>CGGCGGCCGC[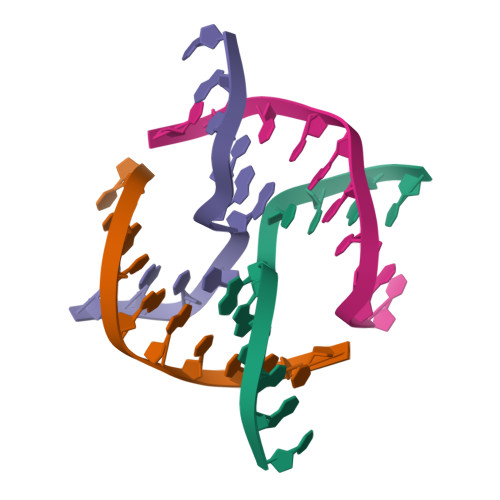4x]>[2x]GPLGSV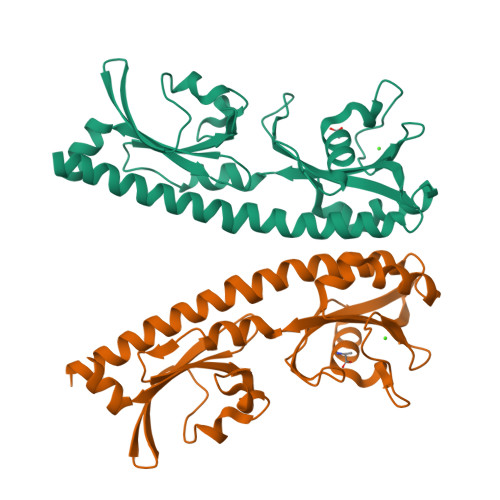REEIESLVQDSLMEMVKGVKNTIESDLASKKGLAQSTTEILQLDPTNKAFAKSVLESPNLKGSFLAIGLGYESDATVVENDDGWEPNADYDPRKRPWYVDAKRERKLVVTEPYVDISTKKIIISIGTPVYQQSNFVGAMFYDVELTQLAQLVNSVNLFDAGYLFITTKDGVTIAHPNAENNGEKFSQFLPNVDLKEGTQRIELDGKYYLVKFAQVPSESWYIGAVVDESIAFAMVDDLRHSSLIHHHHHH>MGSSHHHHHHSSGRENLYFQGHMTFGEQPAYLRVAGDLRKKIVDGSLPPHTRLPSQARIREEYGVSDTVALEARKVLMAEGLVEGRSGSGTYVRERPVPRRVARSGYRPDSGATPFRQEQADGAVRGTWESHSEQAEASGAIAERLDIRPGERVMCTKYVFRDAGEVMMLSTSWEPLAVTGRTPVMLPEEGPVGGMGVVERMAAIDVIVDNVTEEVGARPGLAEELLTLGGVPGHVVLVIQRTYFASGRPVETADVVVP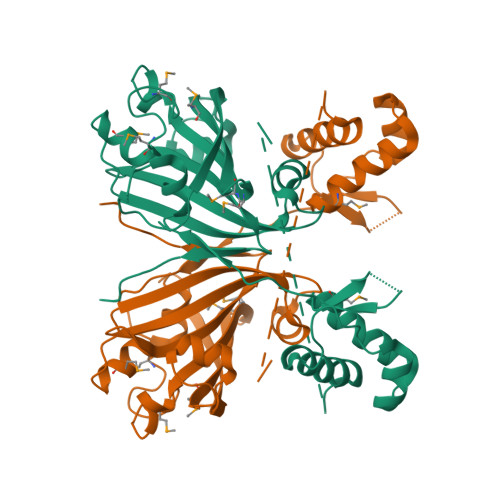ADRYRVAYHLPVK[2x]> XPI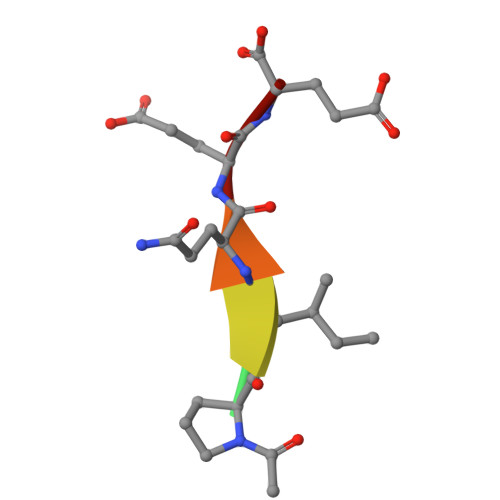QEE>NPCCSHPCQNRGVCMSVGFDQYKCDCTRTGFYGENCSTPEFLTRIKLFLKPTPN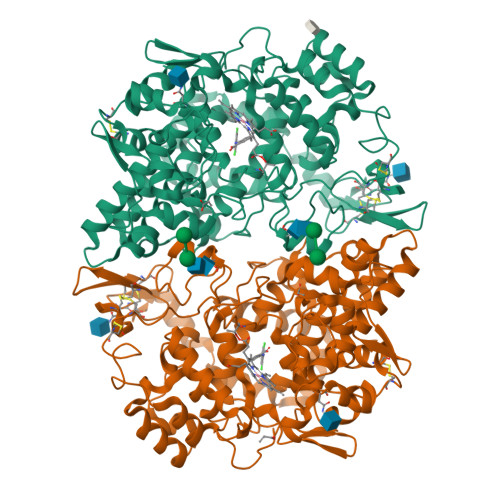TVHYILTHFKGFWNVVNNIPFLRNAIMSYVLTSRSHLIDSPPTYNADYGYKSWEAFSNLSYYTRALPPVPDDCPTPLGVKGKKQLPDSNEIVEKLLLRRKFIPDPQGSNMMFAFFAQHFTHQFFKTDHKRGPAFTNGLGHGVDLNHIYGETLARQRKLRLFKDGKMKYQIIDGEMYPPTVKDTQAEMIYPPQVPEHLRFAVGQEVFGLVPGLMMYATIWLREHNRVCDVLKQEHPEWGDEQLFQTSRLILIGETIKIVIEDYVQHLSGYHFKLKFDPELLFNKQFQYQNRIAAEFNTLYHWHPLLPDTFQIHDQKYNYQQFIYNNSILLEHGITQFVESFTRQIAGRVAGGRNVPPAVQKVSQASIDQSRQMKYQSFNEYRKRFMLKPYESFEELTGEKEMSAELEALYGDIDAVELYPALLVEKPRPDAIFGETMVEVGAPFSLKGLMGNVICSPAYWKPSTFGGEVGFQIINTASIQSLICNNVKGCPFTSFSVP[2x]> MKVEELIIDGFKSYATRTVITDWDPQFNAITGLNGSGKSNILDAICFVLGIASMSTVRASSLQDLIYKRGQAGVTKASVTIVFDNTDKSNSPIGFTNSPQISVTRQVVLGGTSKYLINGHRAPQQSVLQLFQSVQLNINNPNFLIMQGKITKVLNMKPSEILSLIEEAAGTKMFEDRREKAERTMSKKETKLQENRTLLTEEIEPKLEKLRNEKRMFLEFQSTQTDLEKTERIVVSYEYYNIKHKHTSIRETLENGETRMKMLNEFVKKTSEEIDSLNEDVEEIKLQKEKELHKEGTISKLENKENGLLNEISRLKTSLSIKVENLNDTTEKSKALESEIASSSAKLIEKKSAYANTEKDYKMVQEQLSKQRDLYKRKEELVSTLTTGISSTGAADGGYNAQLAKAKTELNEVSLAIKKSSMKMELLKKELLTIEPKLKEATKDNELNVKHVKQCQETCDKLRARLVEYGFDPSRIKDLKQREDKLKSHYYQTCKNSEYLKRRVTNLEFNYTKPYPNFEASFVHGVVGQLFQIDNDNIRYATALQTCAGGRLFNVVVQDSQTATQLLERGRLRKRVTIIPLDKIYTRPISSQVLDLAKKIAPGKVELAINLIRFDESITKAMEFIFGNSLICEDPETAKKITFHPKIRARSITLQGDVYDPEGTLSGGSRNTSESLLVDIQKYNQIQKQIETIQADLNHVTEELQTQYATSQKTKTIQSDLNLSLHKLDLAKRNLDANPSSQIIARNEEILRDIGECENEIKTKQMSLKKCQEEVSTIEKDMKEYDSDKGSKLNELKKELKLLAKELEEQESESERKYDLFQNLELETEQLSSELDSNKTLLHNHLKSIESLKLENSDLEGKIRGVEDDLVTVQTELNEEKKRLMDIDDELNELETLIKKKQDEKKSSELELQKLVHDLNKYKSNTNNMEKIIEDLRQKHEFLEDFDLVRNIVKQNEGIDLDTYRERSKQLNEKFQELRKKVNPNIMNMIENVEKKEAALKTMIKTIEKDKMKIQETISKLNEYKRETLVKTWEKVTLDFGNI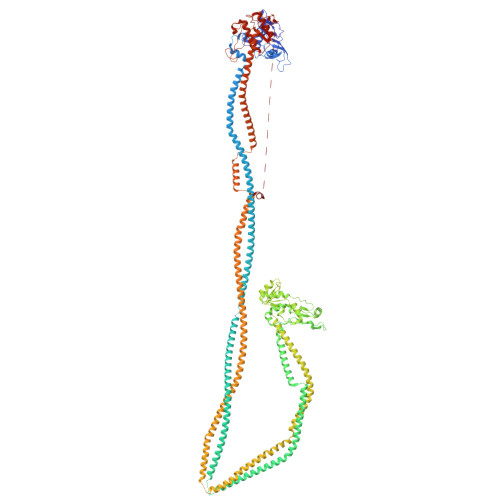FADLLPNSFAKLVPCEGKDVTQGLEVKVKLGNIWKESLIELSGGQRSLIALSLIMALLQFRPAPMYILDEVDAALDLSHTQNIGHLIKTRFKGSQFIVVSLKEGMFANANRVFRTRFQDGTSVVSIMXXXXXXXX>[6x]GENIVFRVISTTGQIPIRDFSADIS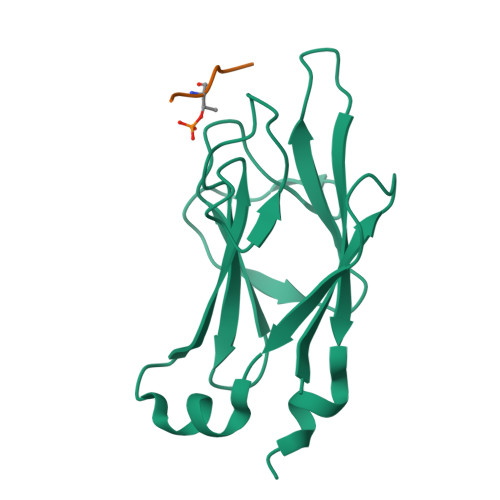QVLKEKRSIKKVWTFGRNPACDYHLGNILPVSNKHFQILLGEDGNLLLNDISTNGTWLNGQKVEKNSYQLLSQGDEITVRTDPTGTILSLVIFINDKFKQSLEQNKVDR;>[6x]KLLPTPPLS> GVALGATRVIYPAGQKQVQLAVTNNDENSTYLIQSWVENADGVKDGRFIVTPPLFAMKGKKENTLRILDATNNQLPQDRESLFWMNVKAIPSMDKSKLTENTLQLAIISRIKLYYRPAKLALPPDQAAEKLRFRRSANSLTLINPTPYYLTVTELNAGTRVLENALVPPMGESTVKLPSDAGSNITYR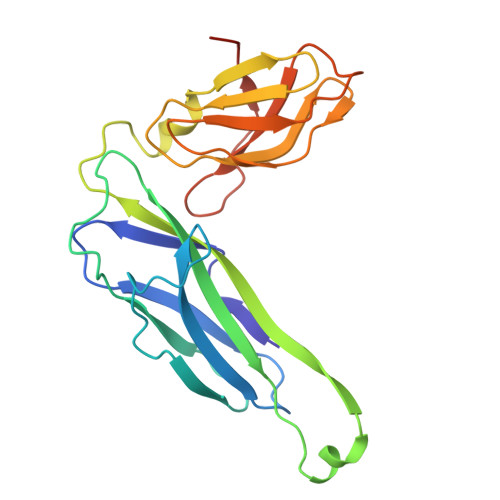TINDYGALTPKMTGVMEHHHHHH> MVQSSVLGFPRMGVLRDLKKANEAYWADKISQEALLAEGKRLRLAHWKIQKDAGVDIIPSNDFAHYDHVLDHIQLFNAVPERYTSQKLSPLDEYFAMGRGHQKGGVDVPALEMVKWFDSNYHYVKPTLQDNQTFSLAKDPKPVREFLEAKEAGFQTRPVLVGPVSFLALGKADRGSSVDPITLLDKLVPVYVELLKQLKAAGAESVQIDEPVLVFDLRPEVKAAFKPAYEAIAAAGDAVPKVVVATYFGDIVHNFDVLPAFSGAAGLHVDLVRNPEQLEPVLKQLGPNQILSAGVVDGRNIWKNDFAKSLEILQTAVKALGSERVIVATSSSLIHTPHTLASEKKLPSDVYEWFSFAVEKVKEVATLAKAVTEPEAVKAELEANAAAIKARTDSKRTNDPAVKERQAQVTPEQHNRKAPFNTRYAEQKKHLSLPLFPTTTIGSFPQTSEIRVQRNKFTKGEISAEEYERFIEKEIELAVKIQDELDLDVYVHGEPERNDMVQYFGERLNGYVFTTHAWVQSYGSRCVRPPIIVGDISRPAPMTVKESKYAASISKKPMKGMLTGPVTCLRWSFPRVDVHQSVQCQQLALALRDEVVDLEKNGIYVIQVDEPALREGLPLRKGQEREAYLKWAVDSFKLATAGVENSTQIHSHFCYSEFQDFFHAIAALDADVLSIENSKSDAKLLKVFIDEEYPRHIGPGVYDIHSPRVPTLEEFKQRIEEMLAYLKPEQLWINPDC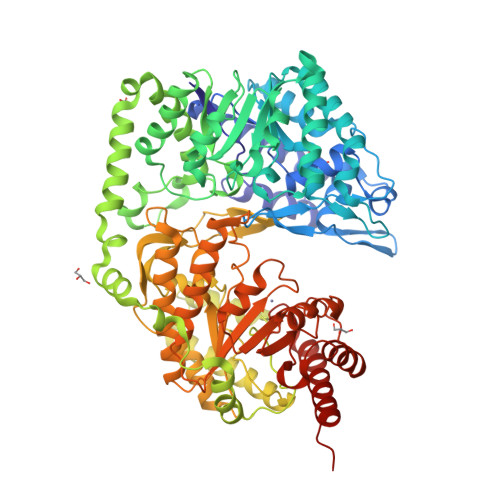GLKTRKWDEVKGALSHMVEAAKYFREKYANKA>MSTVPELLARQVTRAPDAVAVVDRDRVLTYRELDELAGRLSGRLIGRGVRRGDRVAVLLDRSADLVVTLLAIWKAGAAYVPVDAGYPAPRVAFMVADSGASRMVCSAATRDGVPEGIEAIVVTDEEAFEASAAGARPGDLAYVMYTSGSTGIPKGVAVPHRSVAELAGNPGWAVEPGDAVLMHAPYAFDASLFEIWVPLVSGGRVVIAEPGPVDARRLREAISSGVTRAHLTAGSFRAVAEESPESFAGLREVLTGGDVVPAHAVARVRSACPRVRIRHLYGPTETTLCATWHLLEPGDEIGPVLPIGRPLPGRRAQVLDASLRAVAPGVIGDLYLSGAGLADGYLRRAGLTAERFVADPSAPGARMYRTGDLAQWTADGALLFAGRADDQGSHHHHHH[2x];>MTNPFDNEDGSFLVLVNGEGQHSLWPAFAEVPDGWTGVHGPASRQDCLGYVEQNWTDLRPKSLISQISD[2x]

In this work, we have sought to understand the evolutionary history of lipid II targeting glycopeptide antibiotics (GPAs), a vital class of nonribosomal peptides used in the clinic for the treatment of resistant bacterial infections and exemplified by vancomycin (Van) and teicoplanin (Tei). Since ANC1-3 domains display polydisperse elution profiles in size exclusion chromatography, we instead turned to the characterisation of an Acore construct of the Hpg accepting A1 domain from Tei biosynthesis (A1tei), which possesses a homologous pocket to ANC1. The MbtH-like domain Tcp13 also exhibits the anticipated fold, containing a 3-stranded antiparallel β-sheet and an α-helix adjoining the centre of the sheet.

A365 of A1tei is sandwiched between two (W25 and W35) of the three tryptophan residues found in Tcp13. These tryptophan residues, strictly conserved in MbtH-like proteins, are crucial for complex formation, and are located at the end of the second β-strand (W25), in the subsequent loop (W35), and in the C-terminal region behind the first α-helix (W54). The expressed domains were all active, displaying kcat values between 0.08–0.89 min–130, which are comparable to the Tei A1 domain (A1tei).>[2x]MRKIGIIGGTFDPPHYGHLLI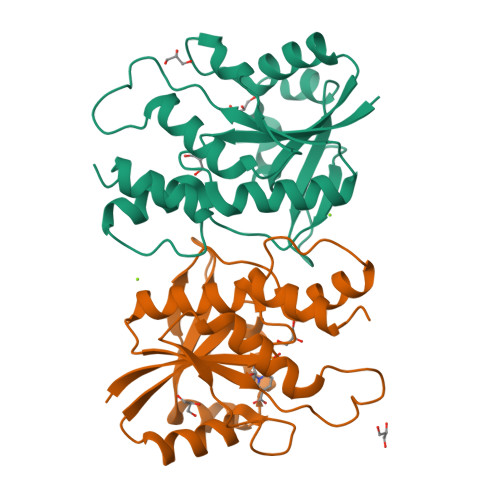ANEVYHALNLEEVWFLPNQIPPHKQGRDITSVESRLQMLELATEAEEHFSICLEELSRKGPSYTYDTMLQLTKKYPDVQFHFIIGGDMVEYLPKWYNIEALLDLVTFVGVARPGYKLRTPYPITTVEIPEFAVSSSLLRERYKEKKTCKYLLPEKVQVYIERNGLYES>[3x]MASQPNSSAKKKEEKGKNIQVVVRCRPFNLAERKASAHSIVECDPVRKEVSVRTGGLADKSSRKTYTFDMVFGAS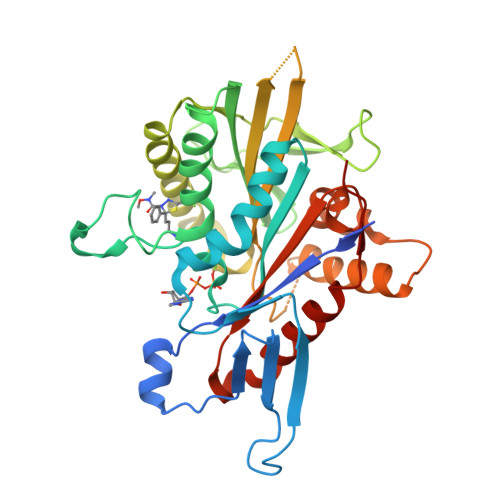TKQIDVYRSVVCPILDEVIMGYNCTIFAYGQTGTGKTFTMEGERSPNEEYTWEEDPLAGIIPRTLHQIFEKLTDNGTEFSVKVSLLEIYNEELFDLLNPSSDVSERLQMFDDPRNKRGVIIKGLEEITVHNKDEVYQILEKGAAKRTTAATLMNAYSSRSHSVFSVTIHMKETTIDGEELVKIGKLNLVDLAGSENIGRSGAVDKRAREAGNINQSLLTLGRVITALVERTPHVPYRESKLTRILQDSLGGRTRTSIIATISPASLNLEETLSTLEYAHRAKNILNKPEVNQK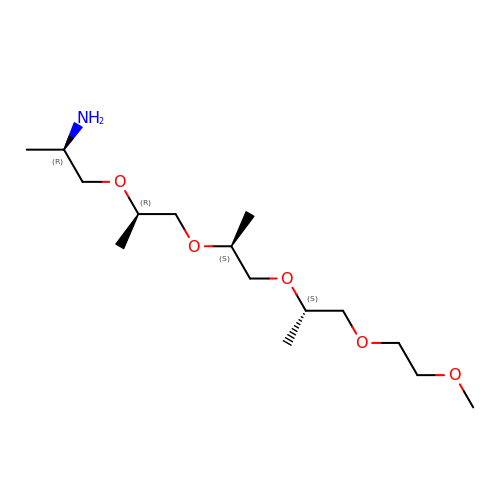(2~{R})-1-[(2~{R})-1-[(2~{S})-1-[(2~{S})-1-(2-methoxyethoxy)propan-2-yl]oxypropan-2-yl]oxypropan-2-yl]oxypropan-2-amine | C15 H33 N O5 | JXGRSFWTZMOYKY-BARDWOONSA-N>[2x]GSMSDGDYDYLIKFLALGDSGVGKTSVLYQYTDGKFNSKFITTVGIDFREKRVVYRANGPDGAVGRGQRIHLQLWDTAGLERFRSLTTAFFRDAMGFLLLFDLTNEQSFLNVRNWISQLQMH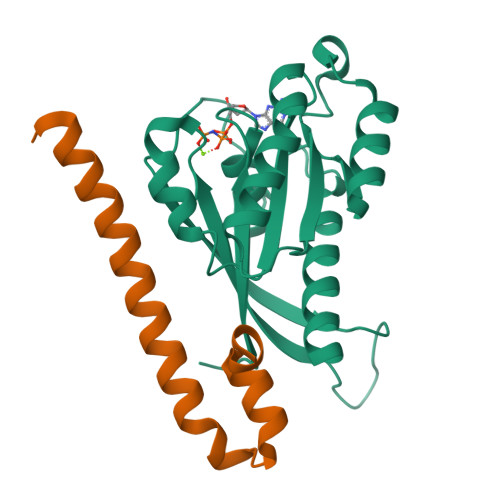AYSENPDIVLCGNKSDLEDQRAVKEEEARELAEKYGIPYFETSAANGTNISHAIEMLLDLIMKRMERSVDKSW;>GSPEFEEQEAIMKVLQRDAALKRAEEERVRHLPEKIKDDQQLKNMSGQWFYEAKAKRHA[2x]> XCRVD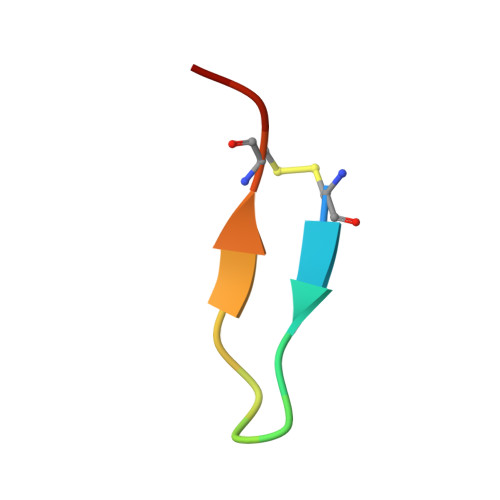LQGWRRCRRX({3-[amino(oxo)acetyl]-1-benzyl-2-ethyl-1H-indol-4-yl}oxy)acetic acid | C21 H20 N2 O5 | 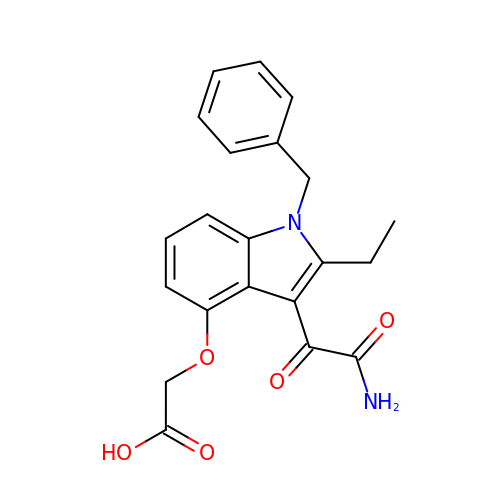BHLXTPHDSZUFHR-UHFFFAOYSA-N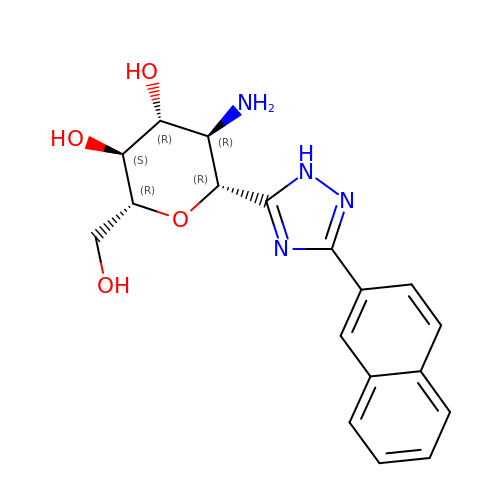(2~{R},3~{S},4~{R},5~{R},6~{R})-5-azanyl-2-(hydroxymethyl)-6-(3-naphthalen-2-yl-1~{H}-1,2,4-triazol-5-yl)oxane-3,4-diol | C18 H20 N4 O4 | IMNCDLXOKIGZHY-OXGONZEZSA-N>[2x]LADAVAHLTPERWEEANRLLVRKALAEFTHERLLTPEREPDDGGGQTYVVRSDDGQTAYRFTATVRALDHWQVDAASVTRHRDGAELPLAALDFFIELKQTLGLSDEILPVYLEEISSTLSGTCYKLTKPQLSSAELARSGDFQAVETGMTEGHPCFVANNGRLGFGIHEYLSYAPETASPVRLVWLAAHRSRAAFTAGVGIEYESFVRDELGAATVDRFHGVLRGRGLDPADYLLIPVHPWQWWNKLTVTFAAEVARGHLVCLGEGDDEYLAQQSIRTFFNASHPGKHYVKTALSVLNMGFMQGLSAAYMEATPAINDWLARLIEGDPVLKETGLSIIRERAAVGYRHLEYEQATDRYSPYRKMLAALWRESPVPSIREGETLATMAS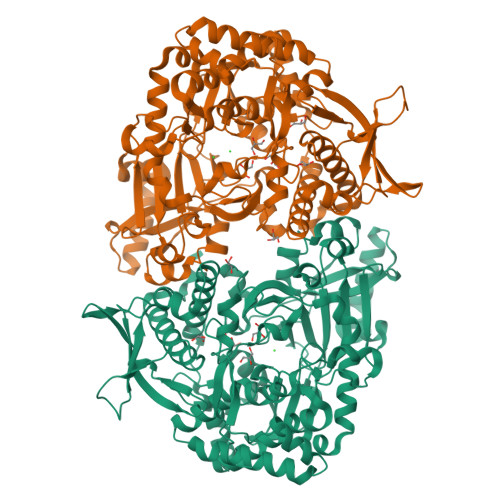LVHQDHEGASFAGALIERSGLTPTEWLRHYLRAYYVPLLHSFYAYDLVYMPHGENVILVLADGVVRRAVYKDIAEEIAVMDPDAVLPPEVSRIAVDVPDDKKLLSIFTDVFDCFFRFLAANLAEEGIVTEDAFWRTVAEVTREYQESVPELADKFERYDMFAPEFALSCLNRLQLRDNRQMVDLADPSGALQLVGTLKNPLAGRG> TNFAVLMAH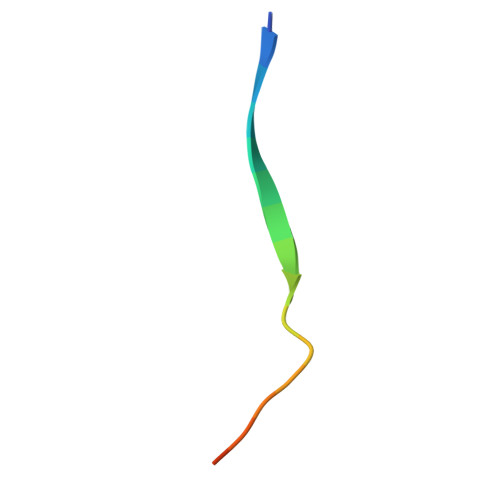REIYHHHHH>[2x]MNNPAIKRIGNHITKSPEDKREYRGLELANGIKVLLISDPTTDKSSAALDVHIGSLSDPPNIAGLSHFLQHMLFLGTKKYPKENEYSQFLSEHAGSSNAFTSGEHTNYYFDVSHEHLEGALDRFAQFFLSPLFDESAKDREVNAVDSEHEKNVMNDAWRLFQLEKATGNPKHPFSKFGTGNKYTLETRPNQEGIDVRQE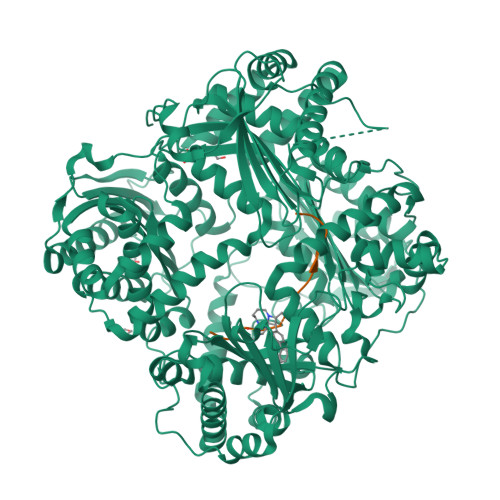LLKFHSAYYSSNLMAVVVLGRESLDDLTNLVVKLFSEVENKNVPLPEFPEHPFQEEHLKQLYKIVPIKDIRNLYVTFPIPDLQKYYKSNPGHYLGHLIGHEGPGSLLSELKSKGWVNTLVGGQKEGARGFMFFIINVDLTEEGLLHVEDIILHMFQYIQKLRAEGPQEWVFQELKDLNAVAFRFKDKERPRGYTSKIAGILHYYPLEEVLTAEYLLEEFRPDLIEMVLDKLRPENVRVAIVSKSFEGKTDRTEEWYGTQYKQEAIPDEVIKKWQNADLNGKFKLPTKNEFIPTNFEILPLEKEATPYPALIKDTAMSKLWFKQDDKFFLPKANLNFEFFSPFAYVDPLHSNMAYLYLELLKDSLNEYAYAAELAGLSYDLQNTIYGMYLSVKGYNDKQPILLKKIIEKMATFEIDEKRFEIIKEAYMRSLNNFRAEQPHQHAMYYLRLLMTEVAWTKDELKEALDDVTLPRLKAFIPQLLSRLHIEALLHGNITKQAALGIMQMVEDTLIEHAHTKPLLPSQLVRYREVQLPDRGWFVYQQRNEVHNNSGIEIYYQTDMQSTSENMFLELFAQIISEPAFNTLRTKEQLGYIVFSGPRRANGIQGLRFIIQSEKPPHYLESRVEAFLITMEKSIEDMTEEAFQKHIQALAIRRLDKPKKLSAESAKYWGEIISQQYNFDRDNTEVAYLKTLTKEDIIKFYKEMLAVDAPRRHKVSVHVLAREMDSNPVVGEFPAQNDINLSQAPALPQPEVIQNMTEFKRGLPLFPLVKPHINFMAAKL;>HSQGTFTSDYSKYLDSRRAQDFVQWLMNT[2x]>MQDCGLPPDVPNAQPALEGRTSFPEDTVITYKCEESFVKIPGEKDSVICLKGSQWSDIEEFCNRSCEVPTRLNSASLKQPYITQNYFPVGTVVEYECRPGYRREPSLSPKLTCLQNLKWSTAVEFCKKKSCPNPGEIRNGQIDVPGGILFGATISFSCNTGYKLFGSTSSFCLISGSSVQWSDPLPECREIYCPAPPQIDNGIIQGERDHYGYRQSVTYACN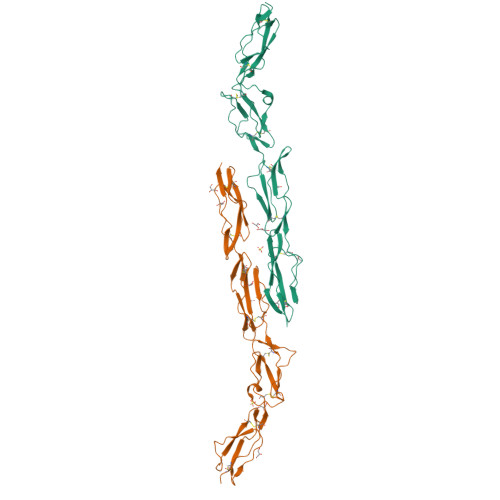KGFTMIGEHSIYCTVNNDEGEWSGPPPECRGC[2x]> MELTPREKDKLLLFTAALVAERRLARGLKLNYPESVALISAFIMEGARDGKSVASLMEEGRHVLTREQVMEGVPEMIPDIQVEATFPDGSKLVTVHNPII;> MIPGEYHVKPGQIALNTGRATCRVVVENHGD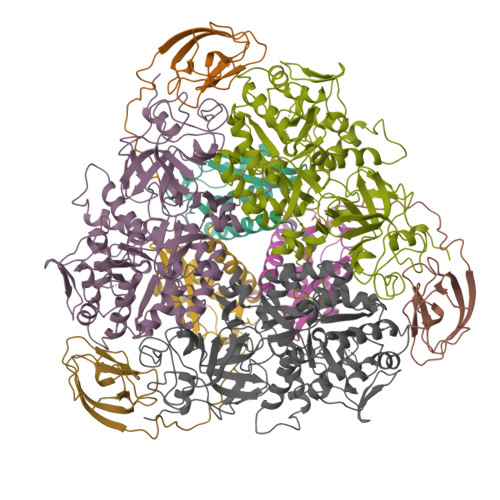RPIQVGSHYHFAEVNPALKFDRQQAAGYRLNIPAGTAVRFEPGQKREVELVAFAGHRAVFGFRGEVMGPL;> SNISRQAYADMFGPTVGDKVRLADTELWIEVEDDLTTYGEEVKFGGGKVIRDGMGQGQMLAADCVDLVLTNALIVDHWGIVKADIGVKDGRIFAIGKAGNPDIQPNVTIPIGAATEVIAAEGKIVTAGGIDTHIHWICPQQAEEALVSGVTTMVGGGTGPAAGTHATTCTPGPWYISRMLQAADSLPVNIGLLGKGNVSQPDALREQVAAGVIGLCIHEDWGATPAAIDCALTVADEMDIQVALHSDTLNESGFVEDTLAAIGGRTIHTFHTEGAGGGHAPDIITACAHPNILPSSTNPTLPYTLNTIDEHLDMLMVCHHLDPDIAEDVAFAESRIRRETIAAEDVLHDLGAFSLTSSDSQAMGRVGEVILRTWQVAHRMKVQRGALAEETGDNDNFRVKRYIAKYTINPALTHGIAHEVGSIEVGKLADLVVWSPAFFGVKPATVIKGGMIAIAPMGDINASIPTPQPVHYRPMFGALGSARHHCRLTFLSQAAAANGVAERLNLRSAIAVVKGCRTVQKADMVHNSLQPNITVDAQTYEVRVDGELITSEPADVLPMAQRYFLF> MSAPNP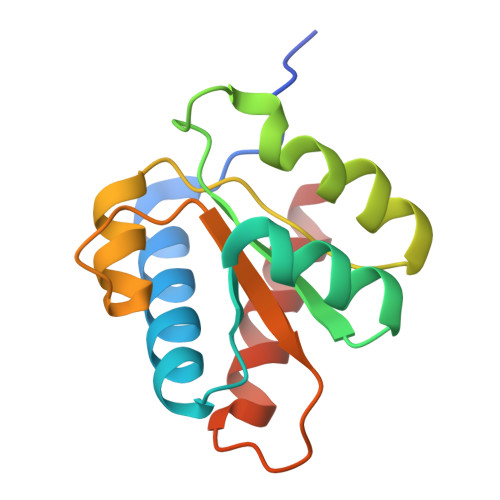KAFPLADAALTQQILDVVQQAANLRQLKKGANEATKTLNRGISEFIIMAADCEPIEILLHLPLLCEDKNVPYVFVPSRVALGRACGVSRPVIAASITTNDASAIKTQIYAVKDKIETLLI>[6x]GSHMEVVNMKAKEIIEFIETFAPKDLAIEGDNIGLQVGDNLDKEIKKLGIALDPSLSVIKKAEKEGVDFLFTHHPLLKDPIRNFTGVIYKKLKILMENDIILYSAHTNLDICKNGLNDALAELY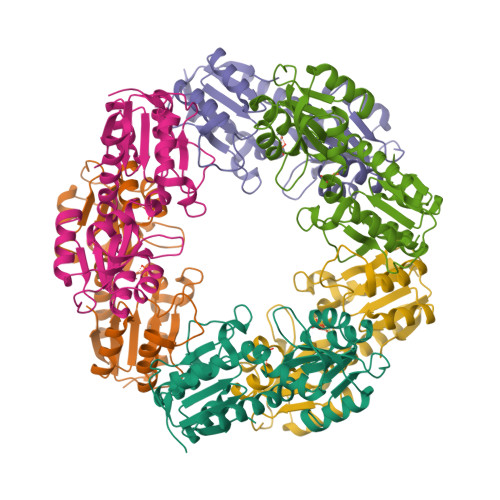NLENPKPLYDNGLGRVGIFKGSFEEFLEITKKYIHKNPIVVKSKEVDDNFKLAVLSGYGLSQSSIKYVAEKADVYLSGDLTHHSKILAEELGLVVVDATHYSTEVFGLKKFKEFLSSNLDLEIISLDF(2R,3S,4R)-3-(4'-chloro-2',6'-difluoro[1,1'-biphenyl]-4-yl)-4-(fluoromethyl)azetidine-2-carbonitrile | C17 H12 Cl F3 N2 | 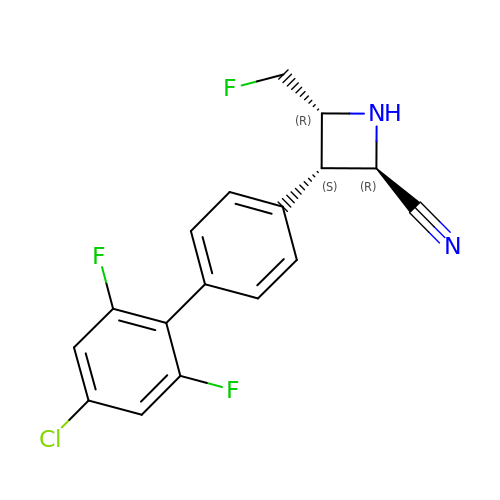XHUZEPHBFHVYMY-YQQAZPJKSA-N> MYGKGKS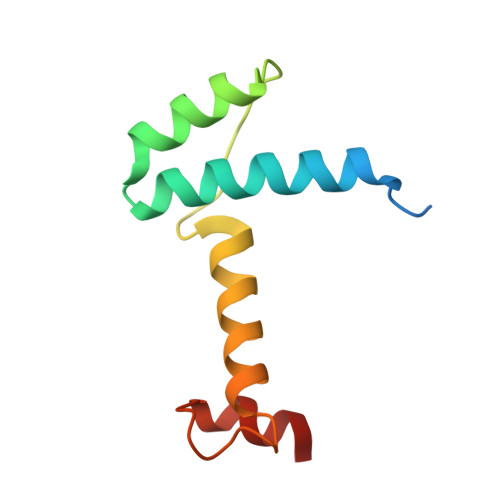NSSAVPSDSQAREKLALYVYEYLLHVGAQKSAQTFLSEIRWEKNITLGEPPGFLHSWWCVFWDLYCAAPERRETCEHSSEAKAFHDY> MIHELLLALSGYPGSIFTWNKRSGLQVSQDFPFLHPSETSVLNRLCRLGTDYIRFTEFIEQYTGHVQQQDHHPSQQGQGGLHGIYLRAFCTGLDSVLQPYRQALLDLEQEFLGDPHLSISHVNYFLDQFQLLFPSVMVVVEQIKSQKIHGCQILETVYKHSCGGLPPVRSALEKILAVCHGVMYKQLSAWMLHGLLLDQHEEFFIKQGPSSGNVSAQPEEDEEDLG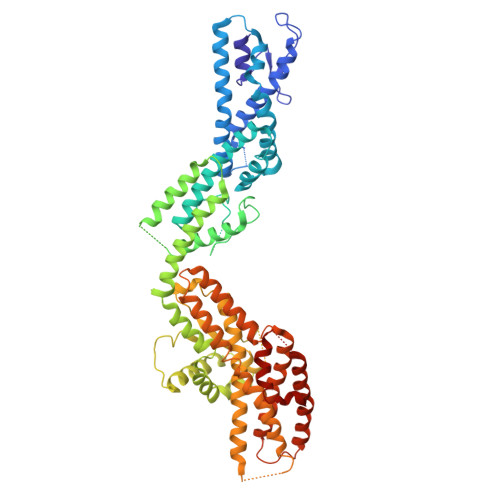IGGLTGKQLRELQDLRLIEEENMLAPSLKQFSLRVEILPSYIPVRVAEKILFVGESVQMFENQNVNLTRKGSILKNQEDTFAAELHRLKQQPLFSLVDFEQVVDRIRSTVAEHLWKLMVEESDLLGQLKIIKDFYLLGRGELFQAFIDTAQHMLKTPPTAVTEHDVNVAFQQSAHKVLLDDDNLLPLLHLTIEYHGKEHKADATQAREGPSRETSPREAPASGWAALGLSYKVQWPLHILFTPAVLEKYNVVFKYLLSVRRVQAELQHCWALQMQRKHLKSNQTDAIKWRLRNHMAFLVDNLQYYLQVDVLESQFSQLLHQINSTRDFESIRLAHDHFLSNLLAQSFILLKPVFHCLNEILDLCHSFCSLVSQNLGPLDERGAAQLSILVKGFSRQSSLLFKILSSVRNHQINSDLAQLLLRLDYNKYYTQAGGTLGSFGM>GPGSEFELPLPEGWEEARDFDGKVYYIDHRNRTTSWIDPRDRYTKPLTFADCISDELPLGWEEAYDPQVGDYFIDHNTKTTQIEDPRVQWRREQEHMLKDYLVVAQEALSAQKEIYQVKQQRLELAQQEYQQLH[2x];>GPGSVAEAPSYQGPPPPYPKHLLHQNPS[2x]

WW domains organize molecular assemblies by binding to short, proline rich peptide motifs each with ~4–6 residues. The type I WW domains bind to a consensus ‘PPxY’ motif (where P is proline, x is any amino acid and Y is tyrosine, also known as PY-motif) with very modest affinities (with Kd in the range of a few to a few tens of µM). To achieve this goal, we determined the high resolustion structures of 7 representative WW tandem/target complexes, and measured the binding constants of >100 WW domain tandems or isolated WW domains binding to known or previously unknown targets. In this study, we discovered that WW tandems, but not individual WW domains, can bind to target proteins with extremely high affinity and with very high sequence specificity.

We also found that the second canonical PY-motif of LATS1 (‘PPPY’) is preceded with an ‘APSY’-motif, and the two motifs are separated by only three residues with the sequence of ‘552QGP554’ (and these two motifs are defined as ‘PY23’). Interestingly, a Gly553Glu mutation of LATS1 was found in patients with renal cell carcinoma. We further found that the KIBRA WW tandem binds to LATS1 PY23 with a Kd of ~0.78 μM, but much more weakly to the canonical PY1 motif (Kd ~78 μM). We solved the high-resolution crystal structures of KIBRA WW tandems in complex with PTPN14 PY12, AMOT PY34 and LATS1 PY23. A residue in the PY-motif linker (R440 in PTPN14, Q282 in AMOT and G553 in LATS) uses its carbonyl group to form a hydrogen-bond with the sidechain of Trp34. Correspondingly, the distances between the two PY motifs of the ligands, measured between the Cα of Tyr in the 1st PY and the Cα of Pro in 2nd PY, are also fixed at ~9.8 Å. The exception is the LATS1 PY23 motifs with the two Cα atoms separated by ~11.5 Å. In contrast, the two PY-motifs of LATS1 are separated by three residues (‘QGP’) and LATS1 binds to the three WW tandems with quite modest affinities. Strikingly, deleting the Gly residue (Gly553) in the three-residue linker of LATS1 PY23 converted the LATS1 mutant (‘LATS1-Δ553’) into a very strong binder of the KIBRA WW tandem (Kd ~17 nM), indicating that a two-residue linker between the two PY-motifs is optimal for specific and high affinity binding to the KIBRA, MAGI2 and MAGI3 WW tandems. The weakened binding of the LATS1-G553E mutant to KIBRA WW12 is likely due to more rigid backbone conformation of Glu over the Glycine residue in the WT protein, such that the defined distance between the two PY-motif binding pockets of KIBRA WW12 can no longer accommodate the LATS1 PY23 mutant.> SNHHRGLASANVDFAFSLYKHLVALSPKKNIFISPVSISMALAMLSLGTCGHTRAQLLQGLGFNLTERSETEIHQGFQHLHQLFAKSDTCLEMTMGNALFLDGSLELLESFSADIKHYYESEVLAMNFQDWATASRQINSYVKNKTQGKIVDLFSGLDSPAILVLVNYIFFKGTWTQPFDLASTREENFYVDETTVVKVPMMLQSSTISYLHDSELPCQLVQMNYCGNGTVFFILPDKGKMNTVIAALSRDTINRWSAGLTSSQVDLYIPKVTISGVYDLGDVLEEMGIADLFTNQANFSRITQDAQLKSSKVVHKAVLQLNEEGVDTAGSTGVTLNLRSKPIILRFNQPFIIMIFDHFTWSSLFLARVMNPV

The hormone binding globulins, corticosteroid binding globulin (CBG) and thyroxine binding globulin (TBG), are examples of naturally occurring site-specific carriers. These hormone carriers release their respective ligands, cortisol in the case of CBG and thyroxine in the case of TBG, when their reactive centre loops are cleaved by elastase, a protease released by neutrophils at sites of inflammation, taking advantage of the site and temporal specificity dictated by neutrophil elastase secretion. Upon cleavage of their reactive centre loops, both hormone binding globulins undergo the canonical serpin conformational change that involves the incorporation of the cleaved reactive centre loop into the central β-sheet A as a new β-strand.

Ser 100 on the s2A/hD loop and Val 236 on the s2B/3B loop of β-sheet B were mutated to cysteines so that under non-reducing conditions, they may be induced to form a disulphide bridge. This forms a direct covalent bond between the s2A/hD loop at the top of helix D and β-sheet B, which along with helices A and H make up the steroid binding pocket. We predicted that by covalently linking the s2A/hD loop to the binding pocket, any effect caused by the movement of the loop as a result of the S-to-R conformational change would be amplified. The disulphide mutations were made on the T349R background to allow cleavage by thrombin. When binding assays were performed at 37°C in the presence of the reducing agent, TCEP, the change in binding affinity of CBG-S100C-V236C-T349R after reactive loop cleavage was very similar to that of wild-type CBG. However, in the absence of TCEP, cleavage of the reactive centre loop resulted in a 6.5-fold decrease in binding affinity for cortisol, as shown in Table 2. We went on to obtain the crystal structure of reactive centre loop-cleaved CBG-S100C-V236C-T349R, which revealed that the binding pocket was indeed perturbed by the presence of the disulphide bridge. Cleavage after Arg349 was supported by clear density for this residue, located at the bottom of sheet A after insertion of the RCL, and for Pro352, located more than 60Å away at the other end of the molecule, though density for Ser350 and Lys351 could not be interpreted unambiguously. The X-ray data also showed that the disulphide linkage has an occupancy of only about half, which suggests either that the disulphide bond is broken by radiation damage during data collection or, more likely, that even under non-reducing conditons, only about half of a given population of the CBG-S100C-V236C-T349R molecules have the desired disulphide bond at a given time. This could explain the relatively small effect of these mutations. (B) When the disulphide bridge is formed, there is an obvious distortion of the steroid binding pocket, as shown here by superimposing the R-state structures of CBG (pale blue, transparent) and CBG-S100C-V236C-T349R (coloured as in A).D-SERINE | C3 H7 N O3 | 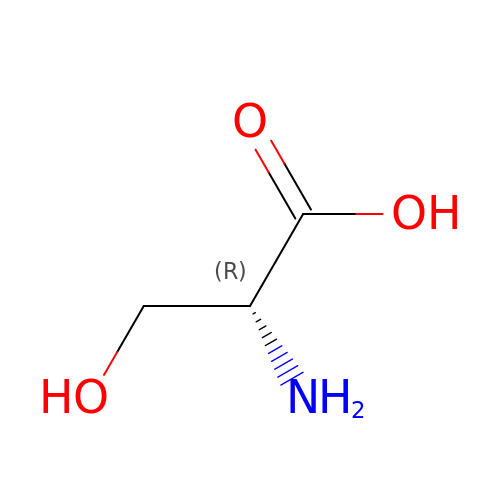MTCFGRXMJLQNBG-UWTATZPHSA-N>[2x]GSSMGMVVE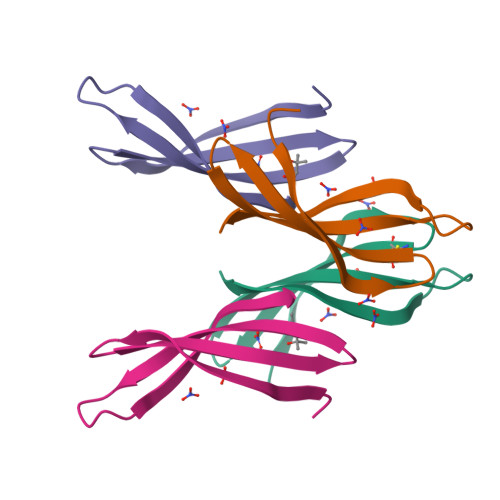ETRDLAETADCVVIEAILVDDGLRYRQLSVGIKDENGDIIRIVPISTVLI N-{4-4-(2,4-DIAMINO-6-OXO-1,6-DIHYDRO-PYRIMIDIN-5-YL)-1-(2,2,2-TRIFLUORO-1,1-DIHYDROXY-ETHYL)-BUT-2-YL-BENZOYL}-GAMMA-GLUTAMYL-GAMMA-GLUTAMYL-GAMMA-GLUTAMYL-GAMMA-GLUTAMYL-GLUTAMIC 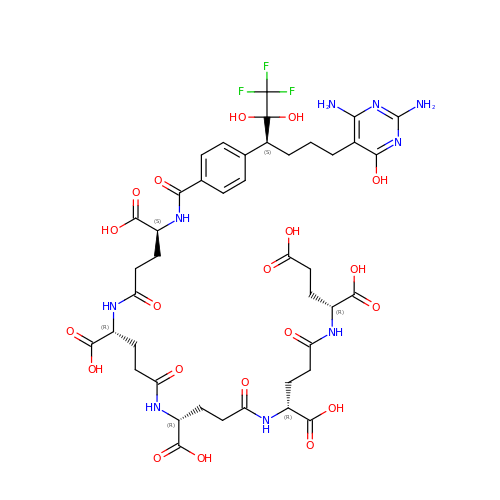ACID | C42 H54 F3 N9 O20 | IWEGOVKIJZGOSL-RCZRCYCLSA-N> MGKKVKKAVKKVTKSVKKVVKEGARPVKQVAGGLAGL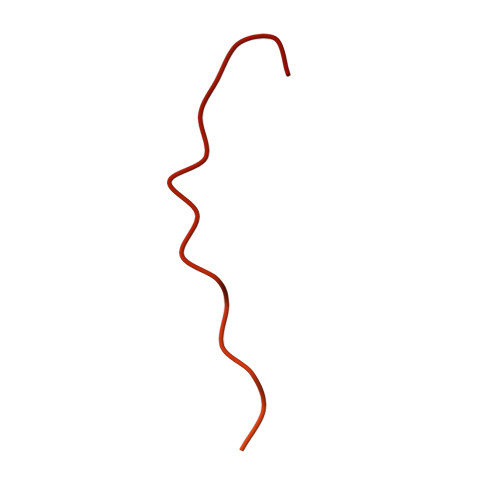AGGTGEAQMVEVPQAAAQIVDVPEKEVSTEDEAQTESGRKKARAGGKKSLSVARSSGGGINI>MVVGWHRPTRLHIDTQAITENVQKECQRLPEGTALFAVVKANGYGHGAVESAKAAKKGGATGFCVALLDEAIELREAGVQDPILILSVVDLAYVPLLIQYDLSVTVATQEWLEAALQQLTPESNTPLRVHLKVDTGMGRIGFLTPEETKQAVRFVQSHKEFLWEGIFTHFSTADEIDTSYFEKQAGRFKAVLAVLEELPRYVHVSNSATALWHPDVPGNMIRYGVAMYGLNPSGNKLAPSYALKPALRLTSELIHVKRLAAGEGIGYGETYVTEAEEWIGTVPIGYADGWLRHL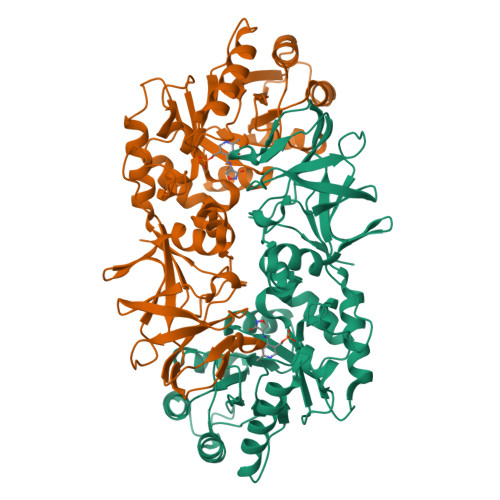QGFTVLVNGKRCEIVGRVCMDQCMIRLAEEVPVGPVVTLVGKDGNEENTLQMVAEKLETIHYEVACTFSQRIPREYN[3x]> IIGGRESRPHSRPYMAYLQIQSPAGQSRCGGFLVREDFVLTAAHCWGSNINVTLGAHNIQRRENTQQHITARRAIRHPQYNQRTIQNDIMLLQLSRRVRRNRNVNPVALPRAQEGLRPGTLCTV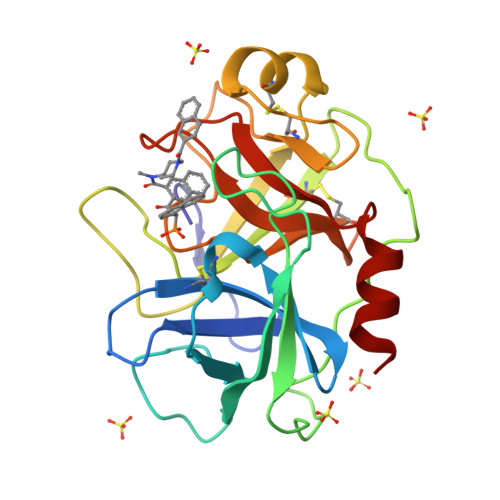AGWGRVSMRRGTDTLREVQLRVQRDRQCLRIFGSYDPRRQICVGDRRERKAAFKGDSGGPLLCNNVAHGIVSYGKSSGVPPEVFTRVSSFLPWIRTTMRS>AENNNLKLASTMEGRVEQLAEQRQVIEAGGGERRVEKQHSQGKQTARERLNNLLDPHSFDEVGAFRKHRTTLFGMDKAVVPADGVVTGRGTILGRPVHAASQDFTVMGGSAGETQSTKVVETMEQALLTGTPFLFFYDSGGARIQEGIDSLSGYGKMFFANVKLSGVVPQIAIIAGPCAGGASYSPALTDFIIMTKKAHMFITGPQVIKSVTGEDVTADELGGAEAHMAISGNIHFVAEDDDAAELIAKKLLSFLPQNNTEEASFVNPNNDVSPNTELRDIVPIDGKKGYDVRDVIAKIVDWGDYLEVKAGYATNLVTAFARVNGRSVGIVANQPSVMSGCLDINASDKAAEFVNFCDSFNIPLVQLVDVPGFLPGVQQEYGGIIRHGAKMLYAYSEATVPKITVVLRKAYGGSYLAMCNRDLGADAVYAWPSAEIAVMGAEGAANVIFRKEIKAADDPDAMRAEKIEEYQNAFNTPYVAAARGQVDDVIDPADTRRKIASALE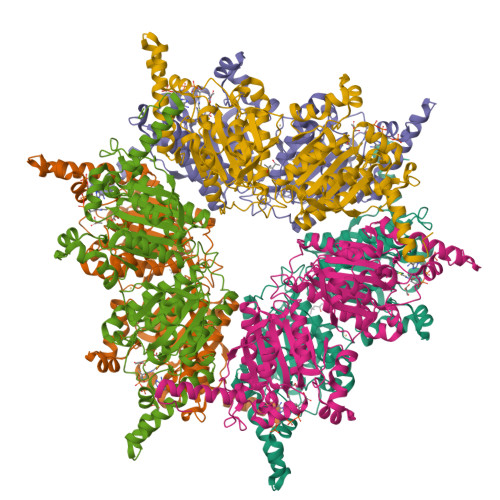MYATKRQTRPAKKHGNFPC[6x]(R)-2-(3-([1,1'-Biphenyl]-4-carbonyl)-3-(4-methylbenzyl)ureido)-3-(((3R,5R,7R)-adamantan-1-ylmethyl)sulfonyl)propanoic acid | C36 H40 N2 O6 S | 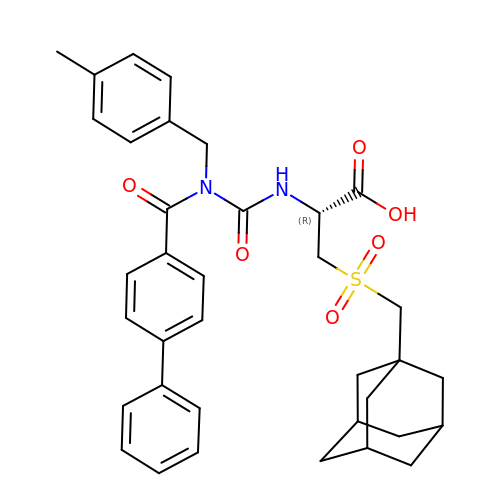OTELSGJQZGOPCK-MGSXHQMGSA-N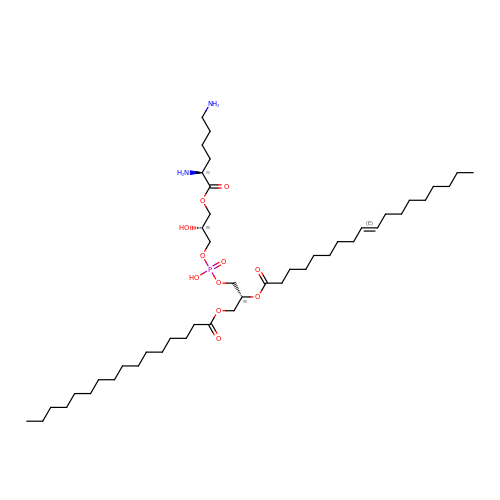[(2R)-1-[[(2R)-3-[(2S)-2,6-bis(azanyl)hexanoyl]oxy-2-oxidanyl-propoxy]-oxidanyl-phosphoryl]oxy-3-hexadecanoyloxy-propan-2-yl] (E)-octadec-9-enoate | C46 H89 N2 O11 P | RAZCYGDQUBGNGD-FLVJYVQPSA-N> GDPVEDIIHDALGSTARRAISSATNVESAANTTPSSHRLETGRVPALQAAETGATSNATDENMIETRCVVNRNGVLETTINHFFSRSGLVGVVNLTDGGTDTTGYVTWDIDIMGFVQLRRKCEMFTYMRFNAEFTFVTTTKNGEARPYMLQYMYVPPGAPKPTGRDAFQWQTATNPSVFVKLTDPPAQVSVPFMSPASAYQWFYDGYPTFGQHPETSNTTYGLCPNNMMGTFAVRVVSREASQLKLQTRVYMKLKHVRAWVPRPIRSQPYLLKNFPNYDSSKITNSARDRSSIKQANM;> SPSVEACGYSDRVAQLTVGNSSITTQEAANIVLAYGEWPEYCPDTDATAVDKPTRPDVSVNRFYTLDSKMWQENSTGWYWKFPDVLNKTGVFGQNAQFHYLYRSGFCLHVQCNASKFHQGALLVAVIPEFVIAGRGSNTKPNEAPHPGFTTTFPGTTGATFHDPYVLDSGVPLSQALIYPHQWINLRTNNCATVIVPYINAVPFDSAINHSNFGLIVIPVSPLKYSSGATTAIPITITIAPLNSEFGGLRQAVSQ;> GIPAELRPGTNQFLTTDDDTAAPILPGFTPTPTIHIPGEVHSLLELCRVETILEVNNTTEATGLTRLLIPVSSQNKADELCAAFMVDPGRIGPWQSTLVGQICRYYTQWSGSLKVTFMFTGSFMATGKMLVAYSPPGSAQPANRETAMLGTHVIWDFGLQSSVSLVIPWISNTHFRTAKTGGNYDYYTAGVVTLWYQTNYVVPPETPGEAYIIAMGADLYKFTLKICKDTDEVTQQAVLQ

Coxsackievirus A10 (CVA10), belonging to the human type-A Enterovirus (HEV-A) subgroup, used to be associated mainly with herpangina, but in recent years has been increasingly reported to co-circulate with other members of the genus such as enterovirus 71 (EV71), CVA16 and CVA6 causing hand, foot, and mouth disease (HFMD) outbreaks in Asia, Europe, and North America2,3. Like most members of the picornavirus family, HEV-As comprise 60 copies of viral proteins VP1, VP2, VP3, and VP4 arranged in pseudo T = 3 symmetry, encasing a positive-sense single-stranded RNA genome. Intriguingly, although CVA10 shares ~69% amino-acid sequence identity with EV71 and CVA16, it utilizes a different receptor, KREMEN1, for entry into host cells, suggesting CVA10 might differ in its mode of entry into host cells or perhaps even in its local structural features that are involved in receptor recognition. Here, we provide models for CVA10 mature virus, empty- and A-particles at atomic resolution, and establish details of the events covering a staged exit of the VP1 N-terminus and ordered structural reorganizations of VP1 GH, VP2 A2B and VP3 GH loops and alterations of viral genome structure as well as genome–capsid interactions during the uncoating.

Compared to mature viruses, the CVA10 empty- and A-particles are markedly expanded with a ~5% increase in capsid radius. In empty particles, there are 60 extra small channels at the base of the canyon (off-axis channels), which are plugged by VP1 and VP2 in A-particle. As expected, both expanded particles lack visible VP4 and harbor neither an hydrophobic pocket nor pocket factor in VP1 due to the movements of the polypeptide backbone in residues 229–233 at the end of the GH loop and the start of strand H, and the conformational changes of the Met229 and Phe232 side chains. Interestingly, only parts of VP1 GH loop (residues 212–223) are flexible in A-particle. Unexpectedly, the A2B loop (residues 38–50) of VP2 located between the twofold axis and the base of the canyon refolds itself from an extended loop observed in the mature virus to a short helix in the A-particle, but is flexible in the empty particle. The most striking differences occur at the VP1 N-terminus (residues 1–71), which lies at the inner surface of the capsid in the mature virus, and is disordered in the empty particle, but traverses the capsid terminating on the external surface at residue 62 in the A-particle (the first 61 residues of VP1 might be disordered). In the empty particle, refolding of the VP1 GH loop and the VP3 GH loop and partial disorder of these two loops as well as the VP2 A2B loop result in the formation of off-axis channels. It is quite likely that the rearrangements of the VP3 GH and VP2 A2B loops, together with increased volume via particle expansion, facilitate the egress of the VP1 N-terminus, obstructing the off-axis channels in A-particle, which might be triggered by receptor-attachment.> GSMIRNKAFVVRLYPNAAQTELINRTLGSARFVYNHFLARRIAAYKESGKGLTYGQTSSELTLLKQAEETSWLSEVDKFALQNSLKNLETAYKNFFRTVKQSGKKVGFPRFRKKRTGESYRTQFTNNNIQIGEGRLKLPKLGWVKTKGQQDIQGKILNVTVRRIHEGHYEASVLCEVEIPYLPAAPKFAAGVDVGIKDFAIVTDGVRFKHEQNPKYYRSTLKRLRKAQQTLSRRKKGSARYGKAKTKLARIHKRIVNKRQDFLHKLTTSLVREYEIIGTEHLKPDNMRKNRRLALSISDAGWGEFIRQLEYKAAWYGRLVSKVSPYFPSSQLCHDCGFKNPEVKNLAVRTWTCPNCGETHDRDENAALNIRREALVAAGISDTLNAHGGYVRPASAGNGLRSENHATLVV

TnpB associates with a single, long RNA (ωRNA) and cleaves double-stranded DNA targets complementary to the ωRNA guide. TnpB from D. radiodurans ISDra2 (hereafter referred to as TnpB for simplicity) consists of 408 residues and has a similar domain organization to Cas12f, which is the smallest subtype among the type V Cas12 enzymes. TnpB adopts a bilobed architecture consisting of recognition (REC) and nuclease (NUC) lobes, which are connected by a linker loop. The REC lobe comprises the wedge (WED) and REC domains, and the NUC lobe consists of the RuvC nuclease domain and the target nucleic acid-binding (TNB) domain.

We reconstituted the ternary TnpB–ωRNA–target DNA complex by mixing the purified TnpB–ωRNA complex and a 35-base pair (bp) double-stranded DNA with phosphorothioate modifications within the DNA backbone around the cleavage site and the TTGAT TAM sequence, and analysed its ternary structure by cryo-EM. We obtained a three-dimensional reconstruction of the ternary complex with an overall resolution of 3.2 Å. The cryo-EM structure revealed that a single TnpB molecule assembles with a single ωRNA molecule to form a ribonucleoprotein effector complex, consistent with the previous molecular mass analysis. The ωRNA–target DNA heteroduplex is accommodated within a central channel formed by the WED, REC and RuvC domains. The TAM-containing DNA duplex (the TAM duplex) is bound to the cleft formed by the WED and REC domains, whereas the ωRNA scaffold binds to a surface formed by the WED and RuvC domains. The TNB domain (residues 327 to 359) is inserted between the β5 strand and the α4 helix and contains a CCCC-type zinc-finger, in which a zinc ion is coordinated by four conserved cysteine residues (C331, C334, C351 and C354). The ωRNA (−116G to 16C) consists of the 16-nt guide segment and 116-nt RNA scaffold, comprising four stems (stems 1–4) and a pseudoknot (PK). The PK coaxially stacks with stem 1 to form a continuous helix. The conserved PK region of the ωRNA is sandwiched between and extensively recognized by the WED and RuvC domains. The TTGAT TAM duplex is recognized by the WED and REC domains.(1R)-1-[3-(cyclohexylmethoxy)phenyl]propane-1,3-diol 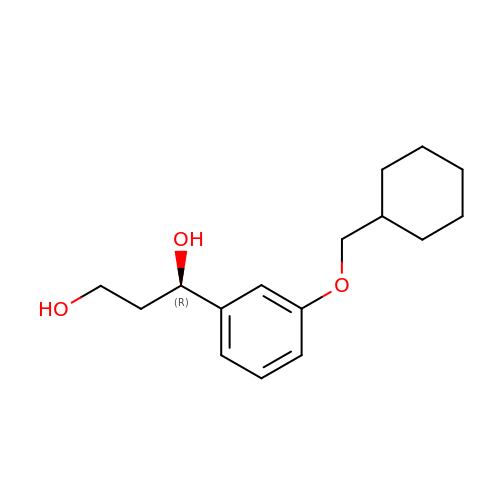| C16 H24 O3 | JEPZJYPEDPLQFU-MRXNPFEDSA-N>MNMLVINGTPRKHGRTRIAASYIAALYHTDLIDLS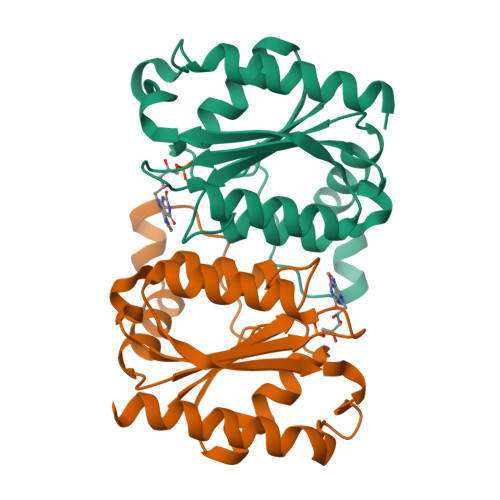EFVLPVFNGEAEQSELLKVQELKQRVTKADAIVLLSPEYHSGMSGALKNALDFLSSEQFKYKPVALLAVAGGGLGGINALNNMRTVMRGVYANVIPKQLVLDPVHIDVENATVAENIKESIKELVEELSMFAKAGNPGV[4x]>MSAFDGVENQMNGPDSSPRLSQDPREPRSLLSSSCFPITLKFVDVCYRVKIHGMSNDSCNIKKLLGLKQKPSDETRSTEERTILSGVTGMISPGEFMAVLGPSGSGKSTLLNAVAGRLHGSNLTGKILINDGKITKQTLKRTGFVAQDDLLYPHLTVRETLVFVALLRLPRSLTRDVKLRAAESVISELGLTKCENTVVGNTFIRGISGGERKRVSIAHELLINPSLLVLDEPTSGLDATAALRLVQTLAGLAHGKGKTVVTSIHQPSSRVFQMFDTVLLLSEGKCLFVGKGRDAMAYFESVGFSPAFPMNPADFLLDLANGVCQTDGVTEREKPNVRQTLVTAYDTLLAPQVKTCIEVSHFPQDNARFVKTRVNGGGITTCIATWFSQLCILLHRLLKERRHESFDLLRIFQVVAASILCGLMWWHSDYRDVHDRLGLLFFISIFWGVLPSFNAVFTFPQERAIFTRERASGMYTLSSYFMAHVLGSLSMELVLPASFLTFTYWMVYLRPGIVPFLLTLSVLLLYVLASQGLGLALGAAIMDAKKASTIVTVTMLAFVLTGGYYVNKVPSGMVWMKYVSTTFYCYRLLVAIQYGSGEEILRMLGCDSKGKQGASAATSAGCRFVEEEVIGDVGMWTSVGVLFLMFFGYRVLAYLALRRIKH[2x]

Abscisic acid (ABA) is a phytohormone essential to the regulation of numerous aspects of plant growth and development. ABCG25 in Arabidopsis thaliana has been identified to be an ABA exporter and play roles in regulating stomatal closure and seed germination. As a ‘half-transporter’ with only one NBD and one transmembrane domain (TMD) in a polypeptide chain, ABCG25 forms a homodimer as a functional unit, similar to other determined ‘half-transporter’ ABCG structures including the human cholesterol transporter ABCG1 (hABCG1) and multidrug transporter ABCG2 (hABCG2)39–47. In this study, we determined the high-resolution structures of ABCG25 in Arabidopsis thaliana in the apo, ABA-bound and ATP-bound states using cryogenic electron microscopy (cryo-EM) single particle analysis.

We also tried to remove CHS during protein purification and extracted the protein from the membrane using DDM alone. The removal of CHS led to dramatically decreased protein yield, indicating a critical role of CHS in stabilizing the protein. Nonetheless, with the purified protein, we obtained an EM map with an overall resolution of 3.7 Å. The protein structure remained almost unchanged compared to that determined with DDM plus CHS extraction, with an RMSD of 0.33 Å. However, in this map, we could still observe the two identical densities in the cavity, further supporting the idea that they are not contributed by CHS. We speculated that they may be some endogenous sterols in Sf9 cells.>MKIMQHSSGFLKLVDDAKSRIQECSVDDIQKMNETQTLDGLL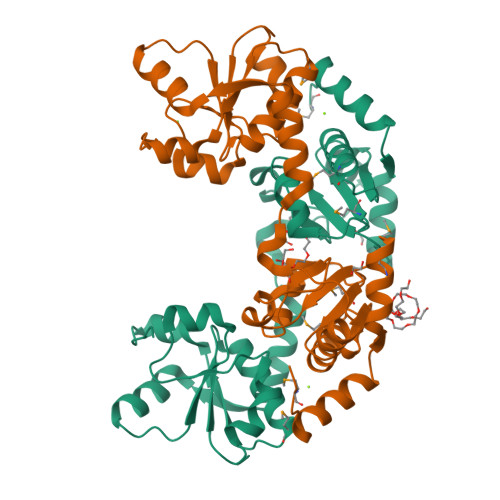IDTREESEVANGYIPNAIHLSKGIIESAIESAVPNKNQKMYFYCGGGFRSALVADKLREMGYKNVISVDGGWRAWNAKGYPTVSPNQFRPNEFLKLVNNAKTQIKECSTTELYNKINSQELDGIVFDVREDSEFNRFHIQGATHLSKGQIEVKIENLVPNKQQKIYLYCGSGFRSALAAESLQHMGYTNVVSIAGGIKDWLANNYPVSQN[2x]> MTKYQGYDVTDATHKTSIHNDWKVVVAKKKPARGVTLTIGIFFDGTGNNRENTASRLMKFNECSAARQGVNQKDAQSCEDFLKEINKNSISNGSYRGYYSNIHWLNILYHPDQVLKKDQTSAQIKTYISGIGTAAGEADSVIGMGLGTSILDIFEGVVTKTDEAMERITQALSEFMGFNLSPDFCIAKIQFDVFGFSRGAAAARHFANRVMEQDPAIARAIAKGLRGDFYDGKPSGEVRFLGLFDTVAAIGGISNFFDINGRSNPGVKLELRPSVAKKVFQITAMNEYRYNFSLNSIKGMWPELALPGAHSDIGGGYNPVGSPLQENESLFLSCPEFEIVSDDTREMDTRVYRKAEQVRKMLMTLPALKHILPHGKLTTKIRSIGVNNSNQRRAGVIQKQVGAAVFFERMAVPNDWANVCLRVMLDAAQEAGVLFEPIRQTNTELQLPSELIFLADKAIAQGKAVRLGQEPQAFTEEELYIIGKYTHCSANWNIESDGNLWVDPTTGEIFIHRFGPKGNKAFVFPNKPNDRWIRSVWYMDDQQRLNDNAVKNTK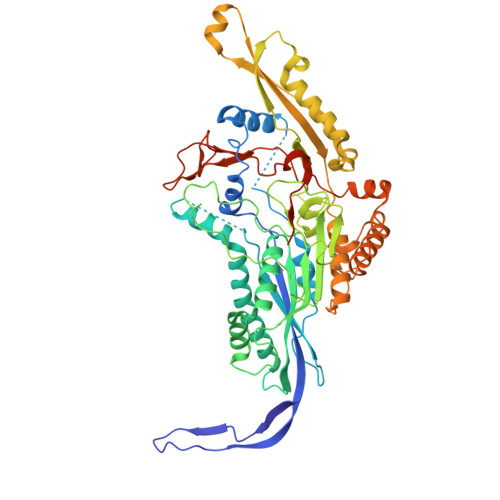VMMSGV> SVGGIISQSFFNGLAGGAASSCEGKGFYTYNAFIAAANAYSGFGTTGSNDVKKRELAAFFANVMHETGGLCYINEKNPPINYCQSSSTWPCTSGKSYHGRGPLQLSWNYNYGAAGKSIGFDGLNNPEKVGQDSTISFKTAVWFWMKNSNCHSAITSGQGFGGTI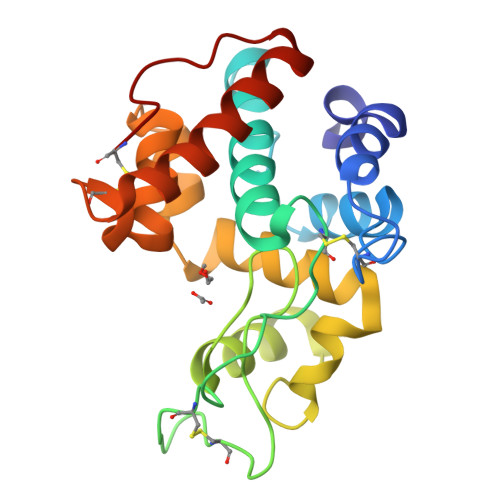KAINSMECNGGNSGEVSSRVNYYKKICSQLGVDPGANVSC> KKVCACPKIL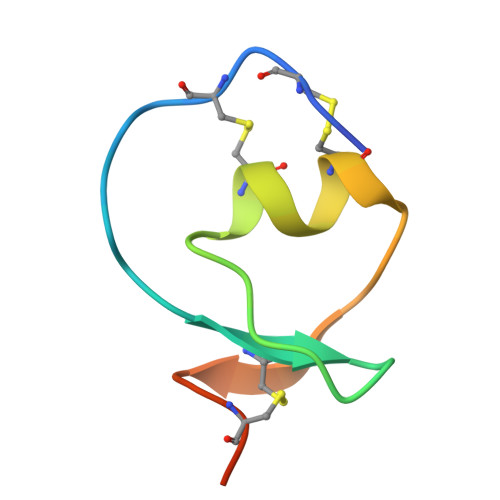KPVCGSDGRTYANSCIARCNGVSIKSEGSCPTGILN> KRGKKHPEP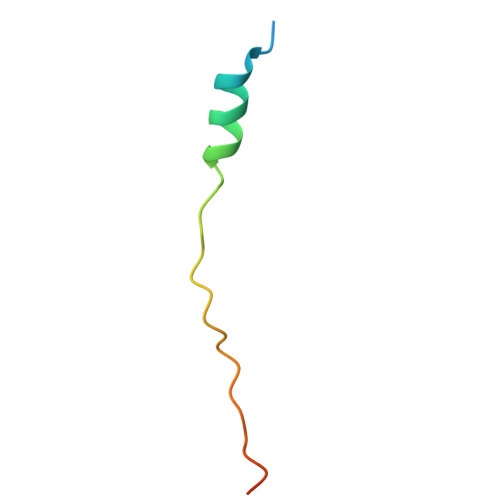VASWMSEQRWAGEPEVMCTLQHKSIAQEAYK> NPISDFP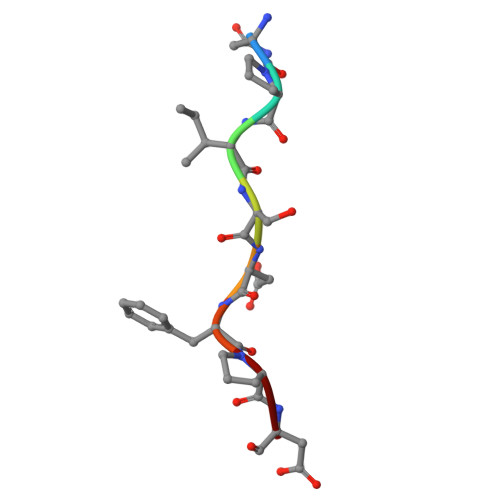D> MGKTRRNRVRNRTDPIAKPVKPPTDPELAKLREDKILPVLKDLKSPDAKSRTTAAGAIANIVQDAKCRKLLLREQVVHIVLTETLTDNNIDSRAAGWEILKVLAQEEEADFCVHLYRLDVLTAIEHAAKAVLETLTTSEPPFSKLLKAQQRLVWDITGSLLVLIGLLALARDEIHEAVATKQTILRLLFRLISADIAPQDIYEEAISCLTTLSEDNLKVGQAITDDQETHVYDVLLKLATGTDPRAVMACGVLHNVFTSLQWMDHSPGKDGACDAILIPTLTRALEHVVPGGAKFNGDARYANITLLALVTLASIGTDFQETLVKGNQGSRESPISAADEEWNGFDDADGDAMDVDQKSSSGEDQEEDYEEIDVKEDDEDDDDDSITSEMQADMERVVGADGTDDGDLEDLPTLRELIQTAVPQLIRLSNLPIDSDESLTIQSHALSALNNISWTISCLEFANGENANIHNAWYPTAKKIWRKTILPILEADSADLKLA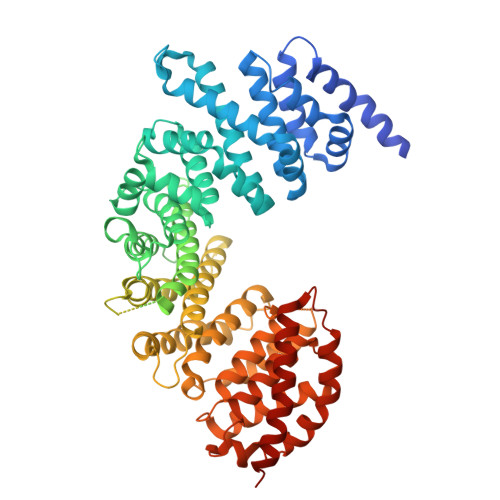TQVTSLAWAVARVLHGETPTDGNPHRKFISLYHSSKQQAGGNSNSIEEPEDPFQGLGVKCIGVVGSLAHDPAPIEVNREVGVFLVTLLRQSNNVPPAEIVEALNQLFDIYGDEELACDKEVFWKDGFLKHLEEFLPKMRTLTKGIDKRTQPELRTRADEALLNLGRFVQYKKKHAPKGSHHHHHH>TSTKRFTCPEESEASNCSCEEFPSKTHFYCPDFNPTLYVDVEDRMRVDFKCYDEPHDFKSLPNLAIGSVKLLTVVDCVLDDDRPILESFKFLEVADVRSFVYNNHENGIRYNAKYFEGMEQLENLTLARGVVSIDRDTFSGFLNLKRLTIEHNKLNLQPGTFEALSNLTYLGLVYNGLNEIQPGLFDGLESLEALSLSYNDIKSLSAGSFNGLSSLRMLNLRVNKIESFDANTFASLKELSRLEITLNPFVSLPRGLFSENKKLKTLILTNNRKLVTLPEELLANLKELTVVNLSHNGVGNLPESLLSGSSGIIELNLGYNRLNSLPEELLSDQPQLQVLNLDHNQLESIPDYFLERNVELQTLYLSHNRLRSLSEKAFTKLKNLKELHLENNQLQTIPQFLFSGTPKLEEIYMQNNQLALHANSFINEELSIADNDNTPFQVLQKLRILHLRNNSISTIFQDWYINNLEMQSLDLSFNKLPGLSYTQLQFQSNITLNLSNNEISQVLLIDDLDLQPYQRINVDLNHNPLNCNCNALKFIQLIQSKAEHGLQFNVDQLRCSEPPNLLDATMDQLQTKDLLCDFESADDCPKDCQCAMRLLDHTVIVNCSGRGLTEFPDLPIPSQLHEDFNALEVHVENNRLTKLPNLTKHNEITQLYARNNSIQNLLPHNIPSKLRIIDLSQNLLKMIDDSTLAQINRSSHLETIRLSQNQWLCDCPASSFLIFVQQNSRLISDMSAIRCHPSGKSLDSITVNELCFEDYTTENLYFQ[2x];>[2x]SDTANAPFLCESEQLLIHPKEELSRNNSMVWIVNTKDYKQGVRIEKCLKRQLGKPCNFCDADTECKQLFHYRTLVAVDKVTKKPYKEQVLLPSCCKCAKILSTGWSHPQFEK

Insect Toll receptors perform critical functions in both embryogenesis and innate immunity. Toll receptors are activated by a complementary family of six cytokine-like molecules called Spaetzle (Spz). Three oligomeric states of the receptor were observed at near-atomic resolutions, suggesting that Toll5A is highly dynamic in the presence of Spz1C.

We observed a ligated heterodimer of Toll5A with a stoichiometry of two receptor ectodomains to one Spz1C ligand (2:1 complex) at a lower resolution (4.2–8.4 Å). The three Toll5A molecules observed are referred to as chain A (teal), chain B (dark blue) and chain C (powder blue) in superimposable conformations in all three structures (RMSD below 2 Å). The Spz1C homodimer is composed of chain D (for distal, in yellow) and chain P (for proximal, in orange), attached to Toll5A chain A at the concave side and to chain B at its “back” or convex side. Nonetheless, Spz1C adopts an asymmetric binding mode, reminiscent of that found in Drosophila despite the lack of sequence conservation, in which chain P contributes about 610 Å2 and chain D, 280 Å2 to the concave binding site. The interactions of Spz1C chain P at the concave site involves mostly residues from the first and third β-strand of Spz1C (Gln-14 and Leu-16, and Tyr-71, respectively) with the LRRNT1 of Toll5A (Tyr-79A, Tyr-65A and His-54A, respectively). Chain D of Spz1C binds extensively to the dimerization interface with over 1,300 Å2 of its accessible surface area, while chain P contributes only 180 Å2, confined to a loop that protrudes from the convex side of LRR14. By contrast in our cryo-EM structure, the β-wings adopt a very different conformation contacting the Z-loop in a pincer-like grasp. Loop structures of Spaetzle1C and Toll5A intercalate, temporarily bridging the receptor C-termini to promote signalling. The dimerization interface of 1480 Å2 is one and a half times the area of the concave binding surface, suggesting a higher affinity binding compared to the concave interface, while the absence of particles with a stoichiometry of 1:1 may indicate a sequential mechanism of assembly in nonequilibrium unsaturated complexes. As there is no possible contact at the dimer interface for the second ligand, we propose that the asymmetric disposition of the receptor chains is the molecular basis of negative cooperativity in the system, where binding of the first ligand in non-saturating conditions makes binding of a second molecule energetically unfavourable.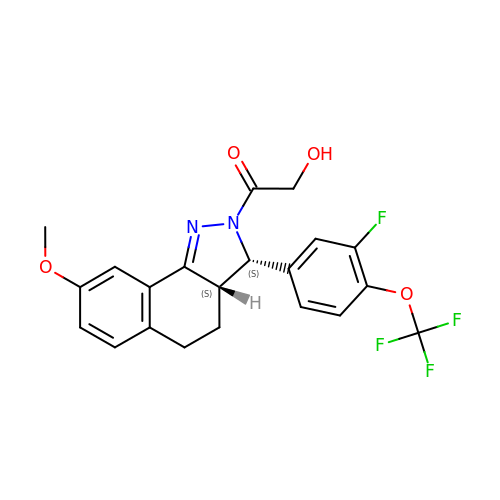1-{(3S,3aS)-3-[3-fluoro-4-(trifluoromethoxy)phenyl]-8-methoxy-3,3a,4,5-tetrahydro-2H-benzo[g]indazol-2-yl}-2-hydroxyethanone | C21 H18 F4 N2 O4 | RPGVJSZQQKMKSB-JLTOFOAXSA-N3-(1-AMINOETHYL)NONANEDIOIC ACID | C11 H21 N O4 | 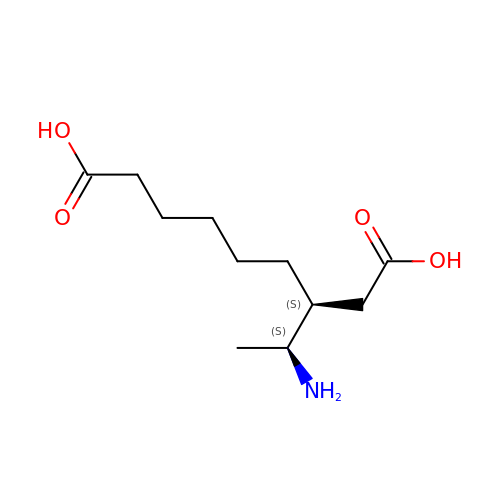NHQUUILSXUJSSP-IUCAKERBSA-N>MLIHIGIDDTDSPNGMCTTYIGAILYREISKIAEPLDFPRLIR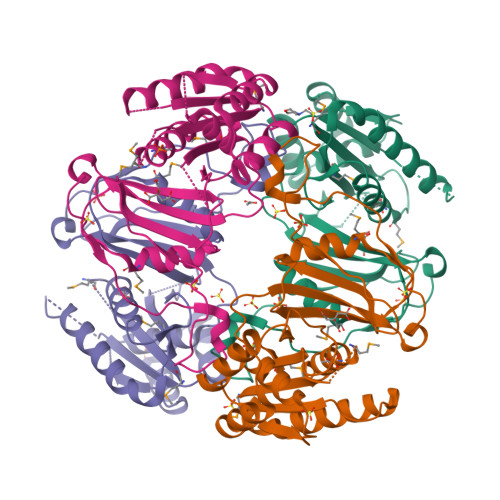LNPNVPYKTRGNGAVAMSFKIDEEKIKEVKTLVIRYVRELADIDHENTNPGIVFLIGEVPKELEEFSLRALREHVTIEEAEHVARKVNAEVYKFKLGRGIIGGLAAIGYPLEKFTYELLAYRKREYWGTPRRVIKESVFYADKWSYPFTYDNVDPYKRTVLITPHGKDPVLVGIRGIDVGKILQVFEMIKIEEPIEFFQVYKTNQNTDD[4x]>[2x]HHGFTTPSRAIAVLSTETIRGNITFTQVQDGKVHVQGGITGLPPGEYGFHVHEKGDLSGGCLSTGSHFNPEHKDHGHPNDVNRHVGDLGNVVFDENHYS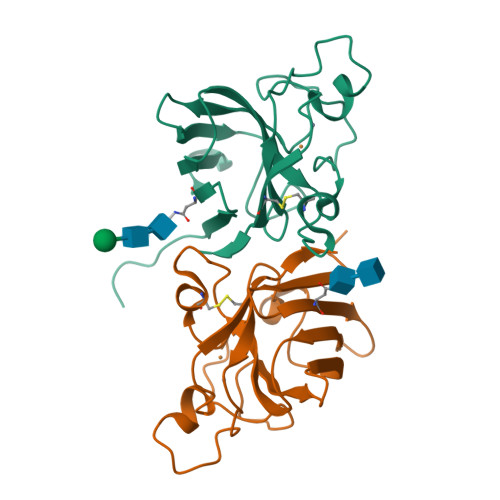RIDLVDDQISLSGPHGIIGRAVVLHEKADDYGKSDHPDSRKTGNAGGRVACGVIGIL> IDKITYPTRIGA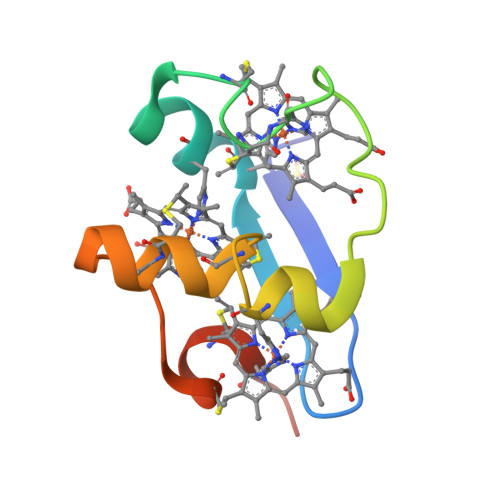VVFPHKKHQDALGECRGCHEKGPGRIDGFDKVMAHGKGCKGCHEEMKIGPVRCGDCHKGGSTH6-(3-methylsulfanylphenyl)sulfanyl-2~{H}-[1,2,4]triazolo[4,3-b]pyridazin-3-one 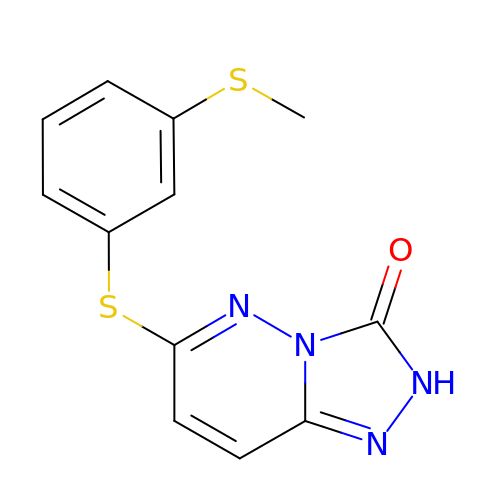| C12 H10 N4 O S2 | VATRPVZFYDKZHK-UHFFFAOYSA-N N-({(2Z)-2-[(2-nitrophenyl)methylidene]hydrazino}carbonothioyl)-beta-D-glucopyranosylamine | C14 H18 N4 O7 S | 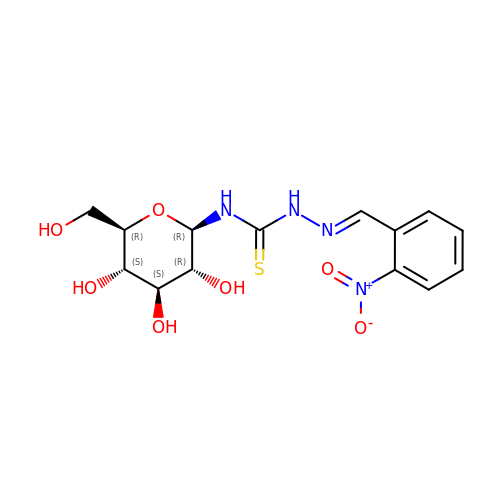HIBBBAGNJNCOKR-ARDSGTFASA-N>MESKRNKPGKATGKGKPVGDKWLDD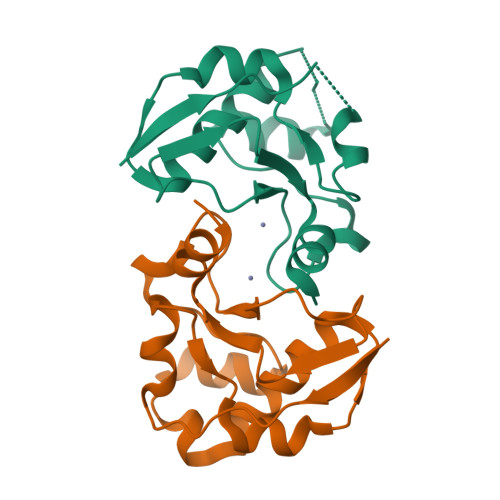AGKDSGAPIPDRIADKLRDKEFKSFDDFRKAVWEEVSKDPELSKNLNPSNKSSVSKGYSPFTPKNQQVGGRKVYELHADKPISQGGEVYDMDNIRVTTPKRHIDIHRGK[2x]> GLPVCAET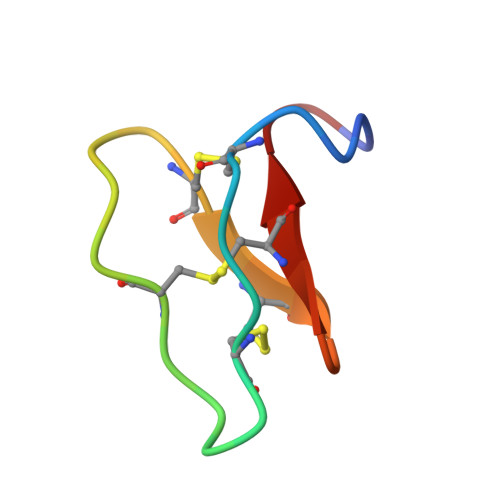CVGGTCNTPGCTCSWPVCTRN>[2x]RSIYLCRHGESELNLRGRIGGDSGLSARGKQYAYALANFIRSQGISSLKVWTSHMK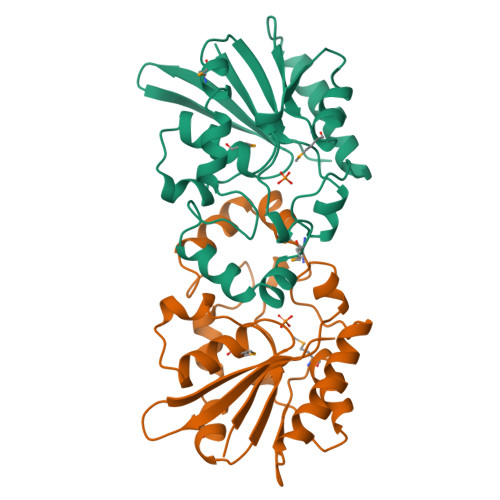RTIQTAEALGVPYEQWKALNEIDAGVCEEMTYEEIQEHYPEEFALRDQDKYRYRYPKGESYEDLVQRLEPVIMELERQENVLVICHQAVMRCLLAYFLDKSSDELPYLKCPLHTVLKLTPVAYGCRVESIYLNV> AGVLLPVAYLGVRALEADPLVLREILLRPKNLELLRNTLGLAAGVLGLATLVALPAAYLTTRTDLRGKRLWATLLTLPLAVPGYVGAYVLLSATGPGGLLPLPRPEGYWGALLVLGLITYPYLFLALRAAFLGVDPSVEEAARTLGHPPWRVFLRVTLPQLLPAFLSGYLVIALHVLGDFGTVSLLRYETFSYAIYLQYSAAFDRVYAAWLALFLLLLTGSLLLLEAALLRRLSLGRTGRGAARTSPPARLGPLAPLAHLFLLLPFLLAVAFPLYALLHLARRFPASATSGLAEALGHALLVALPVAFLSVGMALPIAYLASRYPSAASRTLERLAYLAYAIPPLAYALAWIFFSLRTLPFLYGTLALLVLALALHFLTESLGPVRSALAQVPPRLEEAARTLGDTPTRAFFRVTFPLLWRGAAAGGSLAFIGAMKELPITLLLAPTGFSTLATRVFGYTQEAMFAEAAPFALLIVGLSAAFVGVLLWNERRF;>MERAPLLELKGIRKRFGELEVLRGVDLALYPGEILALLGPSGCGKTTLLRVVAGLEVPDAGRVFLEGRDITALPPEKRGIGFVFQDYALFPHLTALGNVAFGLKGKDRLARARKALERVGMTLFQDRRPGELSGGQQQRVALARALAPGPKLVLLDEPFSSLDAGLRAATREEVRKVLKETGTAALLVTHDQEEALSFADRLGVMRGGEILQVGTPEEVYLRP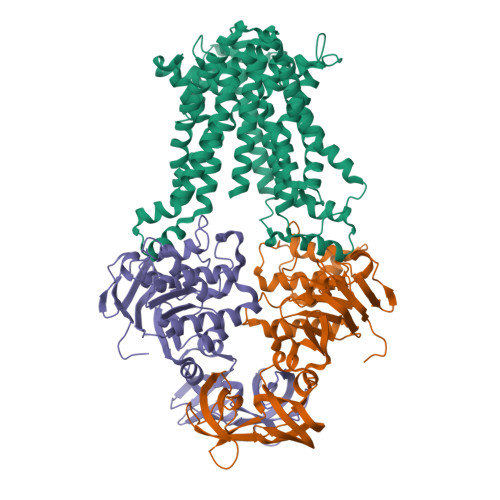KTPFVAQFLGRTNLLPGEGRGRYAETCLGRVPLAEAREGPLLLSLRPEALRLTPPGQGPQGEVVAREFKGHDLTYRVRLHGVQPEREVLVQEGPTCPFKVGDRVGLEVVGEGVALEG[2x]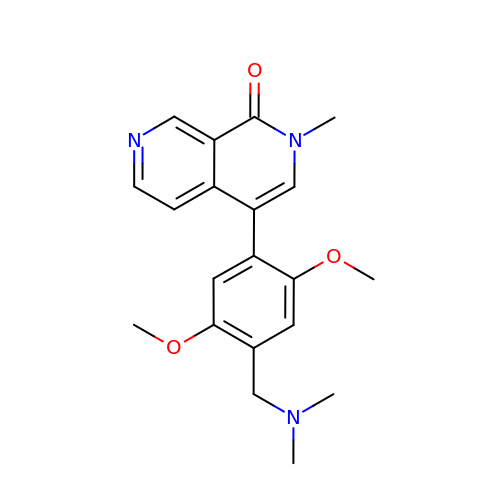4-[4-[(dimethylamino)methyl]-2,5-dimethoxy-phenyl]-2-methyl-2,7-naphthyridin-1-one | C20 H23 N3 O3 | BJFSUDWKXGMUKA-UHFFFAOYSA-N>MSQVGGRGDRCTQEVQGLVHGAGDLSASLAENSPTMSQNGYFEDSSYYKCDTDDTFEAREEILGDEAFDTANSSIVSGESIRFFVNVNLEMQATNTENEATSGGCVLLHTSRKYLKLKNFKEEIRAHRDLDGFLAQASIVLNETATSLDNVLRTMLRRFARDPDNNEPNCNLDLLMAMLFTDAGAPMRGKVHLLSDTIQGVTATVTGVRYQQSWLCIICTMKALQKRHVCISRLVRPQNWGENSCEVRFVILVLAPPKMKSTKTAMEVARTFATMFSDIAFRQKLLETRTEEEFKEALVHQRQLLTMVSHGPVAPRTKERSTVSLPAHRHPEPPKCKDFVPFGKGIREDIARRFPLYPLDFTDGIIGKNKAVGKYITTTLFLYFACLLPTIAFGSLND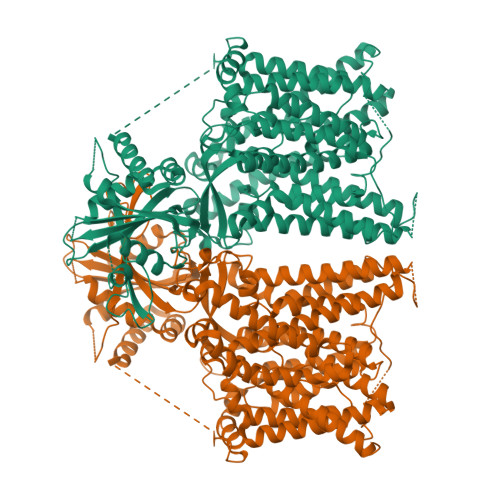ENTDGAIDVQKTIAGQSIGGLLYALFSGQPLVILLTTAPLALYIQVIRVICDDYDLDFNSFYAWTGLWNSFFLALYAFFNLSLVMSLFKRSTEEIIALFISITFVLDAVKGTVKIFWKYYYGHYLDDYHTKRTSSLVSLSGLGASLNASLHTALNASFLASPTELPSATHSGQATAVLSLLIMLGTLWLGYTLYQFKKSPYLHPCVREILSDCALPIAVLAFSLISSHGFREIEMSKFRYNPSESPFAMAQIQSLSLRAVSGAMGLGFLLSMLFFIEQNLVAALVNAPENRLVKGTAYHWDLLLLAIINTGLSLFGLPWIHAAYPHSPLHVRALALVEERVENGHIYDTIVNVKETRLTSLGASVLVGLSLLLLPVPLQWIPKPVLYGLFLYIALTSLDGNQLVQRVALLLKEQTAYPPTHYIRRVPQRKIHYFTGLQVLQLLLLCAFGMSSLPYMKMIFPLIMIAMIPIRYILLPRIIEAKYLDVMDAEHRP[2x]>MELRHLRYFVTVVEEQSISKAAEKLCIAQPPLSRQIQKLEEELGIQLFERGFRPAKVTEAGMFFYQHAVQILTHTAQASSMAKRIATVSQTLRIG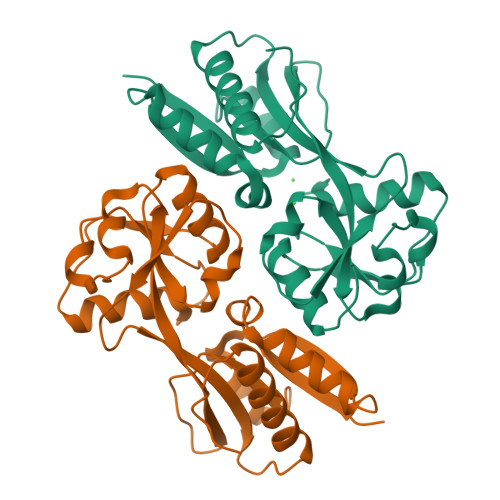YVSSLLYGLLPEIIYLFRQQNPEIHIELIECGTKDQINALKQGKIDLGFGRLKITDPAIRRIMLHKEQLKLAIHKHHHLNQFAATGVHLSQIIDEPMLLYPVSQKPNFATFIQSLFTELGLVPSKLTEIREIQLALGLVAAGEGVCIVPASAMDIGVKNLLYIPILDDDAYSPISLAVRNMDHSNYIPKILACVQEVFATHHIRPLIESILEHHHHHH[2x]> MHYSNIEANESEEERQFRKLFVQLAGDDMEVSATELMNILNKVVTRHPDLKTDGFGIDTCRSMVAVMDSDTTGKLGFEEFKYLWNN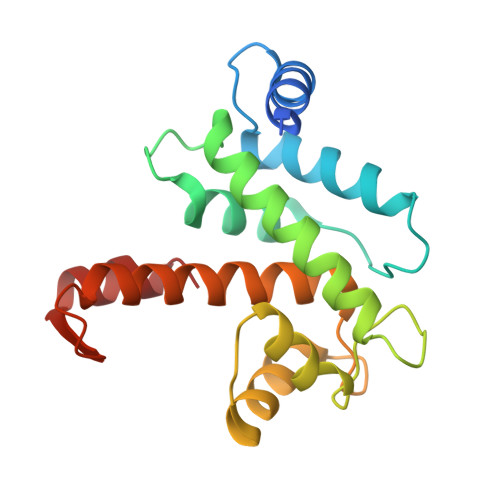IKKWQGIYKRFDTDRSGTIGSNELPGAFEAAGFHLNQHIYSMIIRRYSDETGNMDFDNFISCLVRLDAMFRAFRSLDKNGTGQIQVNIQEWLQLTMYS> MGVIMNQETLIAAVEQMRKLVPALRKVPDETLYAWVEMAELFVCQKTFKDAYVKAIALYALHLAFLDGALKGEDEDLESYSRRVTSFSLSGEF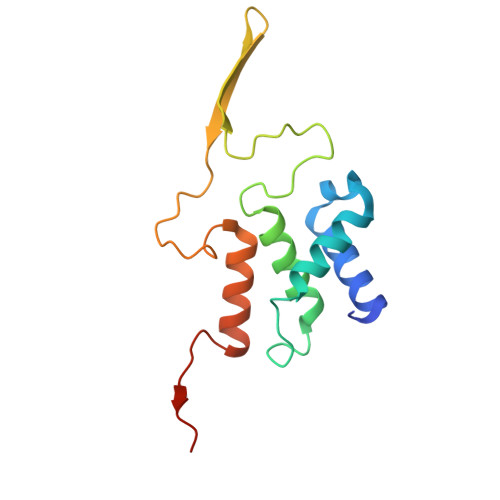SQTFGEVTKNQSGNMMLSTPWGKMFEQLKARRRGRFALMTGLRGGCH>[2x]GAMDKENKKLLCRKCKALACYTADVRVIEECHYTVLGDAFKECFVSRPHPKPKQFSSFEKRAKIFCARQNCSHDWGIHVKYKTFEIPVIKIESFVVEDIATGVQTLYSKWKD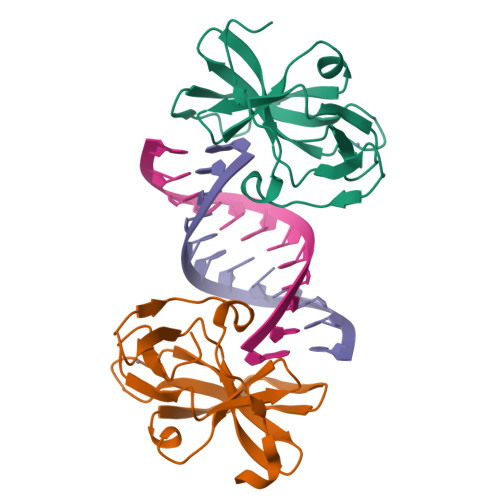FHFEKIPFDPAEMSK>GSSRTSVQTEDDQLIAGQSAGSGSAQLPQEEKAKIAEQVEIFHQEKSKLDAEVAKWDDSGNDIIVLAKQMCMIMMEMTDFTRGKGPLKNTSDVINAAKKIAEA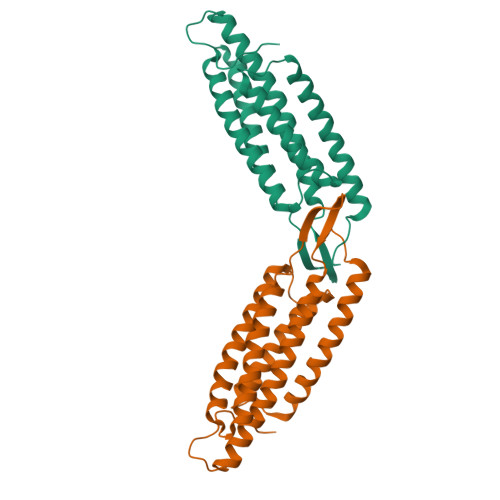GSRMDKLARAVADQCPDSACKQDLLAYLQRIALYCHQLNICSKVKAEVQNLGGELIVSGLDSATSLIQAAKNLMNAVVLTVKASYVASTKYQKVYGTAAVNSPVVSWKMKAPEKKPLVKREKPEEFQTRVRRGSQKKHISPVQALSEFKAMDSF[2x]> MQTVNEMLRRAATRAPDHCALAVPARGLRLTHAELRARVEAVAARLHADGLRPQQRVAVVAPNSADVVIAILALHRLGAVPALLNPRLKSAELAELIKRGEMTAAVIAVGRQVADAIFQSGSGARIIFLGDLVRDGEPYSYGPPIEDPQREPAQPAFIFYTSGTTGLPKAAIIPQRAAESRVLFMSTQVGLRHGRHNVVLGLMPLYHVVGFFAVLVAALALDGTYVVVEEFRPVDALQLVQQEQVTSLFATPTHLDALAAAAAHAGSSLKLDSLRHVTFAGATMPDAVLETVHQHLPGEKVNGYGTTEAMNSLYMRQPKTGTEMAPGFFSEVRIVRIGGGVDEIVANGEEGELIVAASDSAFVGYLNQPQATAEKLQDGWYRTSDVAVWTPEGTVRILGRVDDM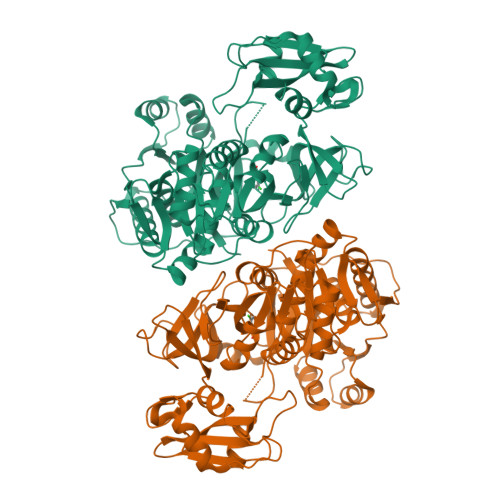IISGGENIHPSEIERVLGTAPGVTEVVVIGLADQRWGQSVTACVVPRLGETLSADALDTFCRSSELADFKRPKRYFILDQLPKNALNKVLRRQLVQQVSS> GDPVKPSRGPLVTCTCESPHCKGPTCRGAWCTVVLVREEGRHPQEHRGCGNLHRELCRGRPTEFVNHYCCDSHLCNHNVSLVLEATQPPSEQPGTDGQ;> NAKGNYCKRTPLYIDFKEIGWDSWIIAPPGYEAYECRGVCNYPLAEHLTPTK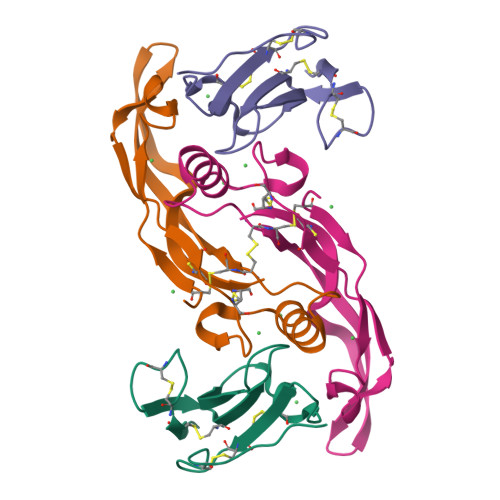HAIIQALVHLKNSQKASKACCVPTKLEPISILYLDKGVVTYKFKYEGMAVSECGCR> AGLTVE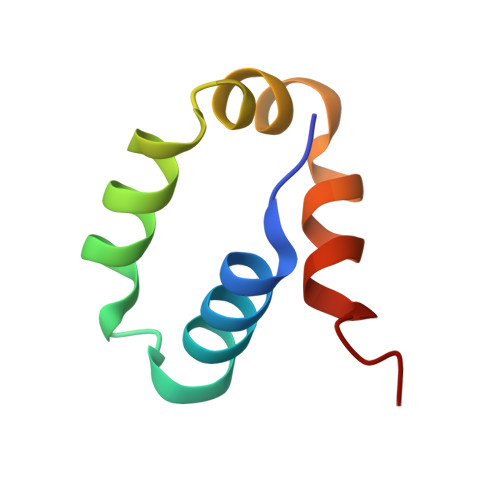DLLSLRQVVSGNPEALAPLLENISARYPQLREHIMANPEVFVSMLLEAVGD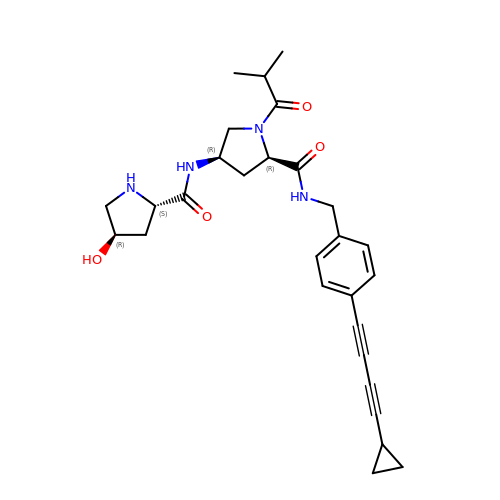(2R,4R)-N-[[4-(4-cyclopropylbuta-1,3-diynyl)phenyl]methyl]-1-(2-methylpropanoyl)-4-[[(2S,4R)-4-oxidanylpyrrolidin-2-yl]carbonylamino]pyrrolidine-2-carboxamide | C28 H34 N4 O4 | YZLBDXYDHITEKM-ZKGSSEMHSA-N The essential enzyme messenger RNA (mRNA) (guanine-N7) methyltransferase catalyzes S-adenosylmethionine (SAM)-dependent conversion of GpppRNA ends to the m7GpppRNA cap structure characteristic of eukaryal mRNAs. The antibiotic sinefungin (SFG) is a SAM analog in which the S-CH3 sulfonium moiety of SAM is replaced by a C-NH2 amine. Available evidence indicates that the antifungal activity of SFG is exerted via inhibition of fungal cap methyltransferase Abd1. Crystal structures of K. lactis and S. cerevisiae Abd1 as binary complexes with SAH or SFG and ternary complexes with GTP•SFG highlight how SFG makes two hydrogen bonds from its C-NH2 amine to the guanine-O6 and -N7 atoms of GTP that account for its higher affinity vis-à-vis SAH and SAM.

A crystal of KlAbd1Δ137 that had been preincubated with 0.7 mM SAH diffracted X-rays to 1.3 Å resolution, was in space group P21 and contained two enzyme protomers in the asymmetric unit. Clear electron densities for SAH were observed in the methyl donor site of both Abd1 protomers. The two protomers in the asymmetric unit are nearly identical and are superimposable with an root mean square deviation (r.m.s.d) of 0.4 Å over 289 Cα positions. KlAbd1Δ137 contains structural motifs that are characteristic of the class 1 methyltransferases, which include a seven-stranded (β1–β5 and β10–β11) central β-sheet surrounded by helices αA–αD, helix αF, and one 310 helix. In addition, KlAbd1Δ137 contains RNA cap methyltransferase-specific structural elements: (i) an α/β domain (aa 281–346) composed of a four-stranded (β6–β9) anti-parallel β-sheet, helix αE, and a 310 helix; and (ii) a C-terminal three helix cluster (helices αG–αI) and a 310 helix, together spanning aa 368–411. In the KlAbd1 crystal structure, SAH occupies the methyl donor site in a conformation similar to that observed previously for SAM, SAH, and aza-SAM in Ecm1 or RNMT and SAH interacts with an ensemble of conserved residues in a manner similar to Ecm1 and RNMT. The adenine base of SAH is sandwiched between the side chains of Ile192 and Phe222 and is partially shielded from the solvent by the side chain of Tyr251. Adenine-N1 and -N6 form hydrogen bonds with the Cys221 amide nitrogen and Asp220-Oδ1, respectively. The ribose O2′ and O3′ atoms form a bidentate hydrogen bond with Asp191-Oδ1 and Oδ2. The SAH amino nitrogen donates hydrogen bonds to the main-chain carbonyl oxygens of Ala169 and Gln246 and makes water-mediated contacts with Glu-Oε2, the Leu168 and Ala169 main-chain carbonyls, and the Gln246 main-chain amide.

>[2x]SPIIKLRNFNNAIKYILIDKFTRAGDVVLELACGKGGDLRKYGAAGISQFIGIDISNASITEALKRYHSMKNLEYQVILITGDCFGESLGVAVESFPECRFPCDIVSCQFALHYAFETEEKARRMLLNVVKSLKIGGYFFGTIPDSEFIRYKMNKIPESVEKPSWGNSIYKVTFSNNEYQKNGNEFPSPFGQMYTFWLEDAIDNVPEYVIPFESFRSLADEYGMELELQKGFNEFFVEEIPNWVNRFSPKMREGLKRSDGRYGVEGVEKEPAAYFYTTFAFRKVRDYQE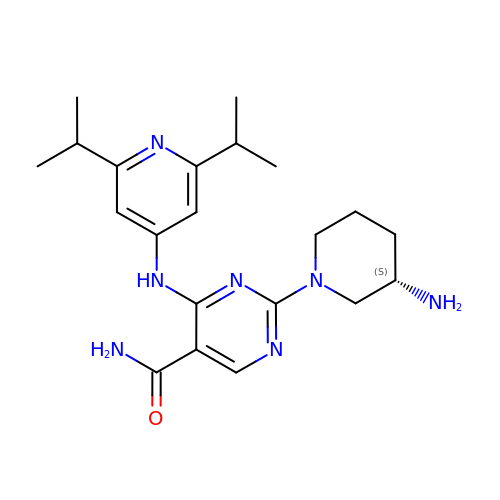2-[(3~{S})-3-azanylpiperidin-1-yl]-4-[[2,6-di(propan-2-yl)pyridin-4-yl]amino]pyrimidine-5-carboxamide | C21 H31 N7 O | BWBUPDTUXQDHSX-AWEZNQCLSA-N> SKVLILFGSSTGNTESIAQKLEELVAAGGHEVTLLNAAEASADNLADGYDAVLMGCSAWGMEDLELQDDFAP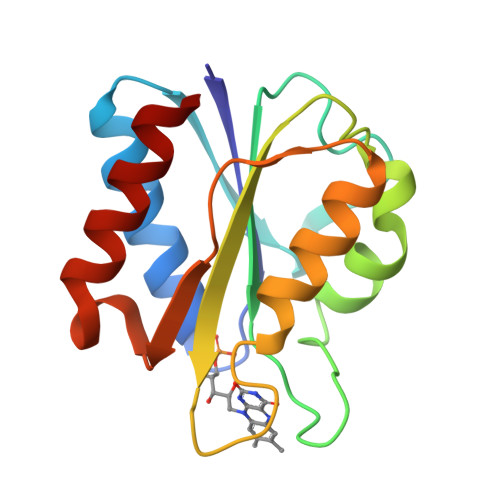LFDEMENMGLKGKKLAAFASGDMEYEHYCGAVPAIEEKARGLGAEVICEGLKIEGDASSDPDAVSAFAEDVLKKL> MSDIRHSLLRRDALSAAKEVLYHLDIYFSSQLQSAPLPIVDKGPVELLEEFVFQVPKERSAQPKRLNSLQELQLLEIMCNYFQEQTKDSVRQIIFSSLFSPQGNKADDSRMSLLGKLVSMAVAVCRIPVLECAASWLQRTPVVYCVRLAKALVDDYCCLVPGSIQTLKQIFSASPRFCCQFITSVTALYDLSSDDLIPPMDLLEMIVTWIFEDPRLILITFLNTPIAANLPIGFLELTPLVGLIRWCVKAPLAYKRKKKPPLSNGHVSNKVTKDPGVGMDRDSHLLYSKLHLSVLQVLMTLQLHLTEKNLYGRLGLILFDHMVPLVEEINRLADELNPLNASQEIELSLDRLAQALQVAMASGALLCTRDDLRTLCSRLPHNNLLQLVISGPVQQSPHAALPPGFYPHIHTPPLGYGAVPAHPAAHPALPTHPGHTFISGVTFPFRPIR;> MSAQGDCEFLVQRARELVPQDLWAAKAWLITARSLYPADFNIQYEMYTIERNAERTATAGRLLYDMFVNFPDQPVVWREISIITSALRNDSQDKQTQFLRSLFETLPGRVQCEMLLKVTEQCFNTLERSEMLLLLLRRFPETVVQHGVGLGEALLEAETIEEQESPVNCFRKLFVCDVLPLIINNHDVRLPANLLYKYLNKAAEFYINYVTRSTQIENQHQGAQDTSDLMSPSKRSSQKYIIEGLTEKSSQIVDPWERLFKILNVVGMRCEWQMDKGRRSYGDILHRMKDLCRYMNNFDSEAHAKYKNQVVYSTMLVFFKNAFQYVNSIQPSLFQGPNAPSQVPLVLLEDVSNVYGDVEIDRNKHIHKKRKLAEGREKTMSSDDEDCSAKGRNRHIVVNKAELANSTEVLESFKLARESWELLYSLEFLDKEFTRICLAWKTDTWLWLRIFLTDMIIYQGQYKKAIASLHHLAALQGSISQPQITGQGTLEHQRALIQLATCHFALGEYRMTCEKVLDLMCYMVLPIQDGGKSQEEPSKVKPKFRKGSDLKLLPCTSKAIMPYCLHLMLACFKLRAFTDNRDDMALGHVIVLLQQEWPRGENLFLKAVNKICQQGNFQY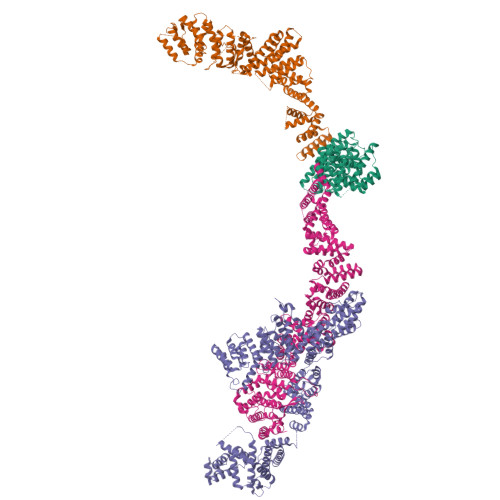ENFFNYVTNIDMLEEFAYLRTQEGGKIHLELLPNQGMLIKHHTVTRGITKGVKEDFRLAMERQVSRCGENLMVVLHRFCINEKILLLQTLT;> MSAEAADREAATSSRPCTPPQTCWFEFLLEESLLEKHLRKPCPDPAPVQLIVQFLEQASKPSVNEQNQVQPPPDNKRNRILKLLALKVAAHLKWDLDILEKSLSVPVLNMLLNELLCISKVPPGTKHVDMDLATLPPTTAMAVLLYNRWAIRTIVQSSFPVKQAKPGPPQLSVMNQMQQEKELTENILKVLKEQAADSILVLEAALKLNKDLYVHTMRTLDLLAMEPGMVNGETESSTAGLKVKTEEMQCQVCYDLGAAYFQQGSTNSAVYENAREKFFRTKELIAEIGSLSLHCTIDEKRLAGYCQACDVLVPSSDSTSQQLTPYSQVHICLRSGNYQEVIQIFIEDNLTLSLPVQFRQSVLRELFKKAQQGNEALDEICFKVCACNTVRDILEGRTISVQFNQLFLRPNKEKIDFLLEVCSRSVNLEKASESLKGNMAAFLKNVCLGLEDLQYVFMISSHELFITLLKDEERKLLVDQMRKRSPRVNLCIKPVTSFYDIPASASVNIGQLEHQLILSVDPWRIRQILIELHGMTSERQFWTVSNKWEVPSVYSGVILGIKDNLTRDLVYILMAKGLHCSTVKDFSHAKQLFAACLELVTEFSPKLRQVMLNEMLLLDIHTHEAGTGQAGERPPSDLISRVRGYLEMRLPDIPLRQVIAEECVAFMLNWRENEYLTLQVPAFLLQSNPYVKLGQLLAATCKELPGPKESRRTAKDLWEVVVQICSVSSQHKRGNDGRVSLIKQRESTLGIMYRSELLSFIKKLREPLVLTIILSLFVKLHNVREDIVNDITAEHISIWPSSIPNLQSVDFEAVAITVKELVRYTLSINPNNHSWLIIQADIYFATNQYSAALHYYLQAGAVCSDFFNKAVPPDVYTDQVIKRMIKCCSLLNCHTQVAILCQFLREIDYKTAFKSLQEQNSHDAMDSYYDYIWDVTILEYLTYLHHKRGETDKRQIAIKAIGQTELNASNPEEVLQLAAQRRKKKFLQAMAKLYF;> MSALCDPPGAPGPPGPAPATHGPAPLSAQELSQEIKAFLTGVDPILGHQLSAREHARCGLLLLRSLPPARAAVLDHLRGVFDESVRAHLAALDETPVAGPPHLRPPPPSHVPAGGPGLEDVVQEVQQVLSEFIRANPKAWAPVISAWSIDLMGQLSSTYSGQHQRVPHATGALNELLQLWMGCRATRTLMDIYVQCLSALIGSCPDACVDALLDTSVQHSPHFDWVVAHIGSSFPGTIISRVLSCGLKDFCVHGGAGGGAGSSGGSSSQTPSTDPFPGSPAIPAEKRVPKIASVVGILGHLASRHGDSIRRELLRMFHDSLAGGSGGRSGDPSLQATVPFLLQLAVMSPALLGTVSGELVDCLKPPAVLSQLQQHLQGFPREELDNMLNLAVHLVSQASGAGAYRLLQFLVDTAMPASVITTQGLAVPDTVREACDRLIQLLLLHLQKLVHHRGGSPGEGVLGPPPPPRLVPFLDALKNHVGELCGETLRLERKRFLWQHQLLGLLSVYTRPSCGPEALGHLLSRARSPEELSLATQLYAGLVVSLSGLLPLAFRSCLARVHAGTLQPPFTARFLRNLALLVGWEQQGGEGPAALGAHFGESASAHLSDLAPLLLHPEEEVAEAAASLLAICPFPSEALSPSQLLGLVRAGVHRFFASLRLHGPPGVASACQLLTRLSQTSPAGLKAVLQLLVEGALHRGNTELFGGQVDGDNETLSVVSASLASASLLDTNRRHTAAVPGPGGIWSVFHAGVIGRGLKPPKFVQSRNQQEVIYNTQSLLSLLVHCCSAPGGTECGECWGAPILSPEAAKAVAVTLVESVCPDAAGAELAWPPEEHARATVERDLRIGRRFREQPLLFELLKLVAAAPPALCYCSVLLRGLLAALLGHWEASRHPDTTHSPWHLEASCTLVAVMAEGSLLPPALGNMHEVFSQLAPFEVRLLLLSVWGFLREHGPLPQKFIFQSERGRFIRDFSREGGGEGGPHLAVLHSVLHRNIDRLGLFSGRFQAPSPSTLLRQGT> LKESPSGYLRSGEGDTGCGELVWVGEPLTLRTAETITGKYGVWMRDPKPTYPYTQETTWRIDTVGTDVRQVFEYDLISQFMQGYPSKVHILPRPLESTGAVMYSGSLYFQGAESRTVIRYELNTETVKAEKEIPGAGYHGQFPYSWGGYTDIDLAVDEAGLWVIYSTDEAKGAIVLSKLNPENLELEQTWETNIRKQSVANAFIICGTLYTVSSYTSADATVNFAYDTGTGISKTLTIPFKNRYKYSSMIDYNPLEKKLFAWDNLNMVTYDI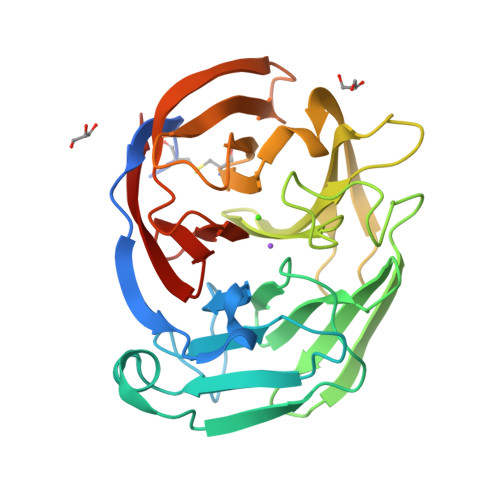KLSKM> GPLGSPEFMLLPNILLTGTPGVGKTTLGKELASKSGLK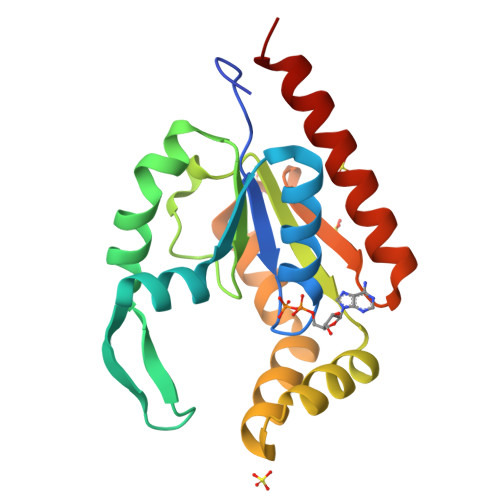YINVGDLAREEQLYDGYDEEYDCPILDEDRVVDELDNQMREGGVIVDYHGCDFFPERWFHIVFVLRTDTNVLYERLETRGYNEKKLTDNIQCEIFQVLYEEATASYKEEIVHQLPSNKPEELENNVDQILKWIEQWIKDHNS> GPGSDKDCEMKRTTLDSPLGKLELSGCEQGLHEIIFLGKGTSAADAVEVPAPAAVLGGPEP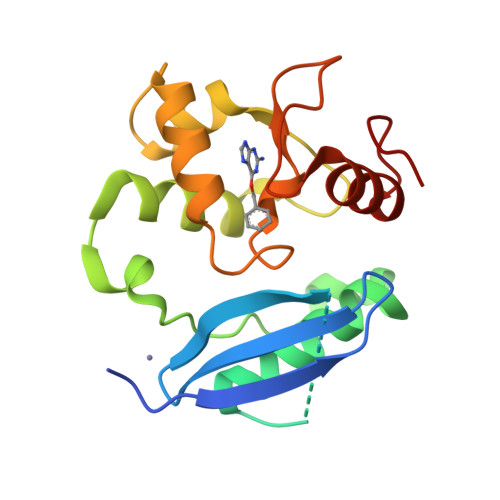LMQATAWLNAYFHQPEAIEEFPVPALHHPVFQQESFTRQVLWKLLKVVKFGEVISYSHLAALAGNPAATAAVKTALSGNPVPILIPAHRVVQGDLDVGGYEGGLAVKEWLLAHEGHRLGKR3-[[4-oxidanyl-1-[(1~{R},2~{R})-2-phenylcyclohexyl]carbonyl-piperidin-4-yl]methyl]quinazolin-4-one | C27 H31 N3 O3 | 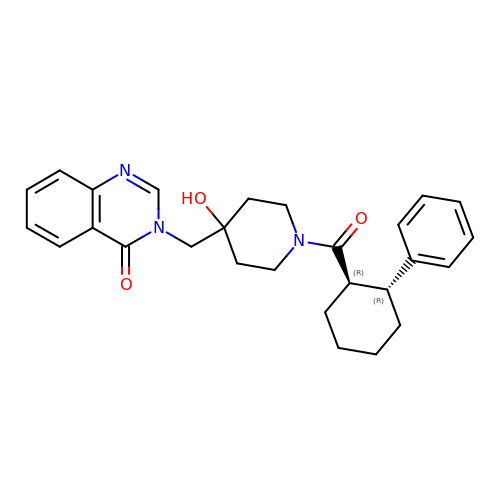FPRPKRNRTCFBRF-FCHUYYIVSA-N>GAMAMNGEAICSALPTIPYHKLADLRYLSRGASGTVSSARHADWRVQVAVRHLHIHTPLLDSERKDVLREAEILHKARFSYILPILGICNEPEFLGIVTEYMPNGSLNELLHRKTEYPDVAWPLRFRILHEIALGVNYLHNMTPPLLHHDLKTQNILLDNEFHVKIADFGLSKWRMMSLSQSRSSKSAPEGGTIIYMPPENYEPGQKSRASIKHDIYSYAVITWEVLSRKQPFEDVTNPLQIMYSVSQGHRPVINEESLPYDIPHRARMISLIESGWAQNPDER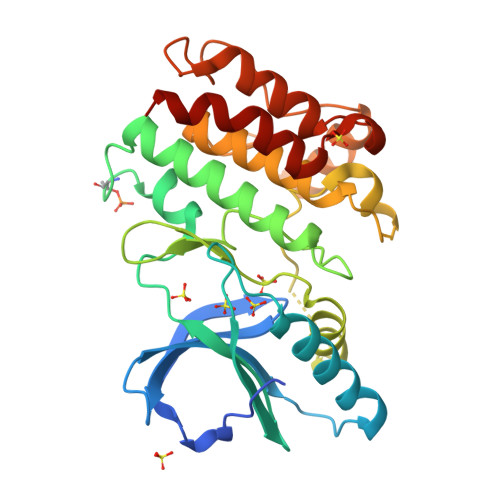PSFLKCLIELEPVLRTFEEI[4x]>[2x]MDKELGKTLRRLRQGKQVSISSLADEHLSKSQISRFERGESEISSSRLLNLLDKLNITIDEFVSTHSKTHTHFFTL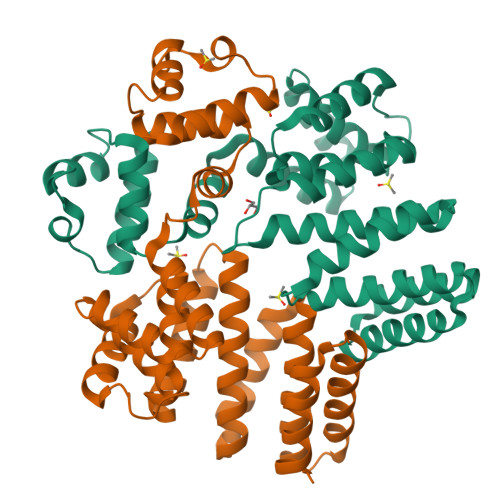LSRVRKYYAEKNVAKLLKLLEDYAHKDYESTMIKAILSSIEPTVEPSEEEVTRLTDYLFSVEQWGYYEIILLGNCSRFINYNTLFLLTKEMVTSFAYSEQNKTNKTLVTQLSINCLIISIDYSYFDHSHYLIEKIEFLLRDELNFYEKTVFLYVHGYYKLKQGQVSGKDDMRQALQIFKYLGEDALYYSYKEHYRKEVLGDEEDEEEG>[4x]SMPKLPENYTDETWQKLKEAVEAIQNSTSIKYNLEELYQAVENLCSYKISANLYKQLRQICEDHIKAQIHQFREDSLDSVLFLKKIDRCWQNHCRQMIMIRSIFLFLDRTYVLQNSMLPSIWDMGLELFRAHIISDQKVQNKTIDGILLLIERERNGEAIDRSLLRSLLSMLSDLQIYQDSFEQRFLEETNRLYAAEGQKLMQEREVPEYLHHV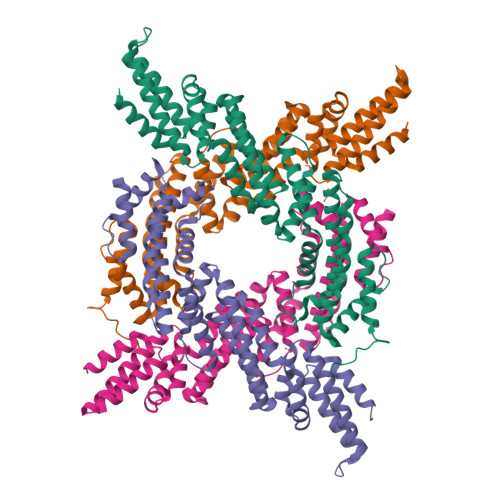NKRLEEEADRLITYLDQTTQKSLIATVEKQLLGEHLTAILQKGLNNLLDENRIQDLSLLYQLFSRVRGGVQVLLQQWIEYIKAFGSTIVINPEKDKTMRQELDDFKDKVDHIIDICFLKNEKFINAMKEAFETFINKRPN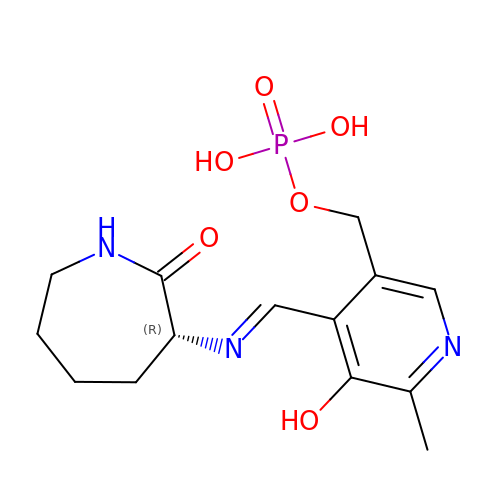[6-methyl-5-oxidanyl-4-[(~{E})-[(3~{R})-2-oxidanylideneazepan-3-yl]iminomethyl]pyridin-3-yl]methyl dihydrogen phosphate | C14 H20 N3 O6 P | QOFJUFQRGNVZPX-KOSUEXCASA-N>[2x]MGSSHHHHHHSSGRENLYFQGHMIPEHLSIYTAYNANIAAIVKLNQETIQNLINAFDPDEVKRRIEEYPREINEPIDFVARLVHTLKLGKPAAVPLVNEKMNEWFDKTFRYEEERLGGQAGIIANTLAGLKIRKVIAYTPFLPKRLAELFKKGVLYPVVENGELQFKPIQEAYREGDPLKINRIFEFRKGLKFKLGDETIEIPNSGRFIVSARFESISRIETREDI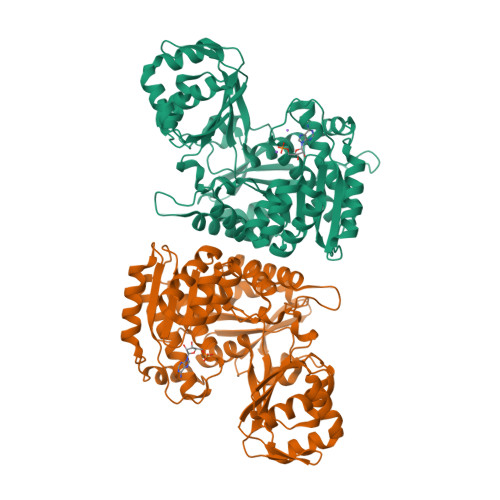KPFLGEIGKEVDGAIFSGYQGLRTKYSDGKDANYYLRRAKEDIIEFKEKDVKIHVEFASVQDRKLRKKIITNILPFVDSVGIDEAEIAQILSVLGYRELADRIFTYNRLEDSILGGMIILDELNFEILQVHTTYYLMYITHRDNPLSEEELAKSLEFGTTLAAARASLGDIRGPDDYKVGLKVPFNERSEYVKLRFEEAKSRLRMREYKVVVIPTRLVQNPVLTVGLGDTISAGAFLTYLEFLKRHGS>MMYKEPFGVKVDFETGIIEGAKKSVRRLSDMEGYFVDERAWKELVEKEDPVVYEVYAVEQEEKEGDLNFATTVLYPGKVGKEFFFTKGHFHAKLDRAEV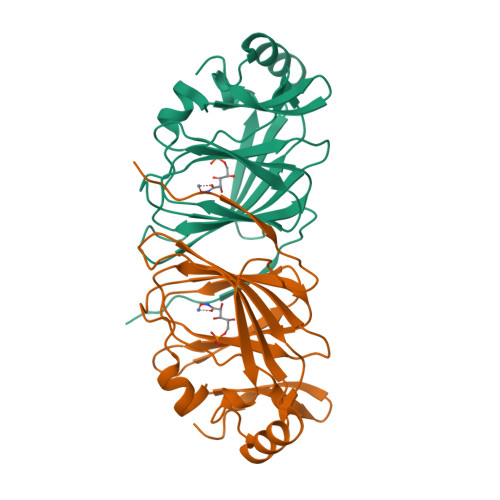YVALKGKGGMLLQTPEGDAKWISMEPGTVVYVPPYWAHRTVNIGDEPFIFLAIYPADAGHDYGTIAEKGFSKIVIEENGEVKVVDNPRW[2x]> GIGAVLKVLTTGLPA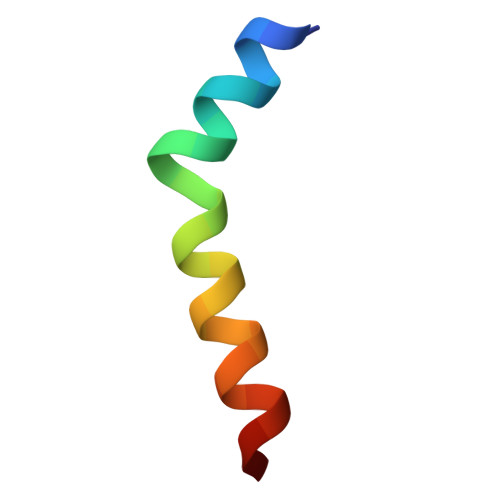LISWIKRKRQQX>SNARVFNFAAGPATLPENVLLKAQADLYNWRGSGMSVMEMSHRGKEFLSIIQKAESDLRQLLEIPQEYSVLFLQGGATTQFAALPLNLCKSDDTVDFVVTGSWGDKAVKEAKKYCKTNVIWSGKSEKY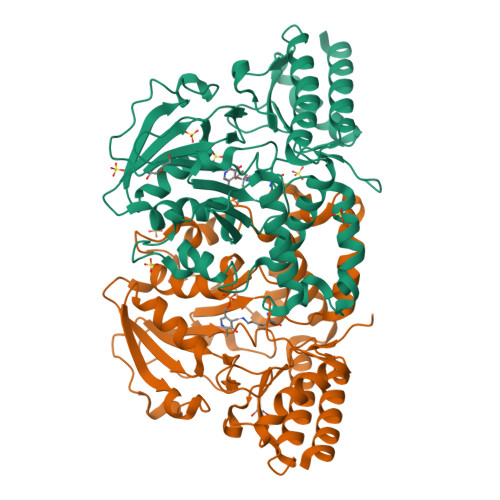TKVPSFEELEQTPDAKYLHICANETIHGVEFKDYPVPKNGFLVADMSSNFCSKPVDVSKFGVIYGGAQKNVGPSGVTIVIIRKDLIGNAQDITPVMLDYKIHDENSSLYNTPPCFGIYMCGLVFEDLLEQGGLKEVEKKNQRKADLLYNAIEESNGFFRCPVEKSVRSLMNVPFTLEKSELEAEFIKEAAKEKMVQLKGHRSVGGMRASIYNAMPLAGVEKLVAFMKDFQAKHA[4x]>GSHMQQVNPDFIEALTEKITEEVTAKVTEELTKQNMEFFAAVAKQSQDNFDRINKRLEERDE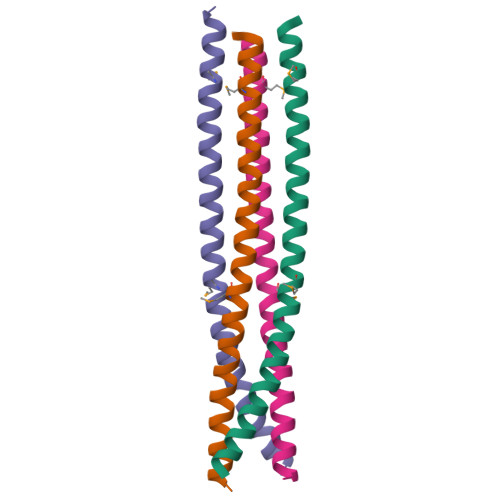KLMSTIRLIQEQKSANAQ[4x]> MDPRETAIGLVRYVTENAAKDFDGESIAAIIYRLRVVENYVSSDVDIICEAMRILIKKLVNLPPITFSPDVWMPIMTSITEGAIEPQWRIMMESIDISKFSSTSSNFVHMDSITASSTKCSEQITSICKGFALEFGLTRRLFSAIWNTDLEETARKMMNQEWDSVKIDSSPDSAKQAAGLIEKSIFDLFSEMKDHETFANELYYAALARILNNSRRLQENKKPAIQDSEDISFYESSLHIYDELIKKLWPHLSKKDPNVKKNTLIIFEKLISLSPTDVLVQRITEKFIDSCEWLKISGEEICTSMEPRLWKIVGSLVSRILDLKKTIPYEIVSYAIAVHITQEVTLASPEVSDCGPDSFDSTCDQPSNMKERFLRHMVDSYFQTRSSLLSIIQFLRTAKSSEEIVQFMRVFYPELVFGNETLITHAAIEMLRESASHHSIKADDFISIVLSVIDAPAIVRIIDVISCIKDEKVRKEAVEKTIIRMANDLEDEDQKREGYVNHLHENGSFWNDIAKYADASILDKAGKRFVEVSVDSMDIRSSVLATDIFLTILKLKLTSEAEREPESCVICNVSYSNIKIDLEKWNKMGNILVECNMVKRSKSEALPLFTIHQLENIDLPMRDLVYVVTQMKFLDTKEGMELHRKFYDGLPGVNVIFEKFMSKSHKIELCMKLLDEFAKIIAINEKSLIFSLDHENILDWLEEIGVLDSPQITEKLVDICFSIEVWDVLTLLQLDGPECHYWDLQMFGRFWKTSLMDLLDEKMMKKVNEKMGSILKEQYDKQSHVAKATREKRSNGKFPNRPKVADWEEQLLLMHNRIAGHLTKKKVEDFADESTQKFTWLLGVCSGQMSYKKEVAVDAEKILSRLYPDAEKRNEVLYHFGVSSILKGLDRPRGKLSLHILFMQIYLDLVQIDSKSWKIDDSVQKLSRRLGGFNEWLMIVDEEKREDDGGFRIYIVLNLSHYFWELLEGCKASQVVDAHAILKIRKFAEVLASILDKITFWPNPKLHAYYYIAQFLEPLETIFHFPEIAEQNRKVIESFFKQLFDKLLEQKYQEGLLQDTKLIIQKTDKYLSSSLNLFNEYNTQEPSKIYPVNEIFSLFCRYGSENVHLYCLKMIKKSLQTLASNILEHEHILKGEVCIETELQKRLVCDAVLLTEFFGYFSCIYAQVSENQPSEHDDVAKAFMLLDSDIHLKTKSRKRSTQNSVAVGSHRHQTAENMDLNFCTYKSTGRAYVTQHWYNCYTCNMMESEGVCSVCAINCHRGHDLAYSKKGSFFCDCGEKKCGAMQGIYHLPNSMYSLRGQLPEKNGDKTLPKIRNVFEHRFENLNSNCCDELKSALNDVQEEFKEVQDDLEQILEAVDFANQKALQVTEERLAVLESFNDMDDVIISEKEKFIEPLESGHFLPTRRDDLPVQELRVASSQHKIRELSDIIKLDDGTELLVLIPESIQTCLQLHYMDTRTNLIQGMHALRTETEQIPFNARSLHVSGNRLVVCGQYEFFALRFSPQGDVIDRAHIKLLENGASSSMNNNPVVRAKFCREIESDKRRRQLIAVATMQYIRIYDLTLHETNFVEEMVLPAGNVEDVEIINQEDGNVRILVLSSSGYLYEHNISVFNAENNSIFLTNVVNTPGMDMNGDGVSLHYSSTFNLLFVSLENGAFVAQLPEPTGNSTAPIYDWKHLNIKNPVDAWKETSGIIACLSTNCNHQVNYFHPTVGKILLQKTSVKRSIMTYFLMTSAKNQSVYSVLIYPNVPTCEIWETSWNNVHDLWIDDVPTERYAVEVVEQKSTQIPIDRDELVLLAEQCEQIRTVDWNCREIGMFYTHEELNNRLSSSDSLPITLIQQTHFKLSARITNFRQIVRMIRVEVEGNTGPEYLKIGTTRYSISSRGPKTFDLRLSREESLALDHRDITIEVIPRSNQNRVTLKSLRLLGCDRSAMDEIQPRYERQPILTNSNKLVYSILEFATLSGLEWAGNMAKKHLSRKLNHPAVCSVSTRAIVKCHPSVDEELFKIIDGAYLQEWKALIDWTESEGFGEMRLHHVEQLLDRMEAVRTRWPYFVKSLKREFGTVTSFVELMRNEMKRMPLHRCQMMAQAIVKIVFGLLSNGTNEAEQLIHVFLNIFTDQDTYHLANDMRSAVQETISRFENALKEEKKLMVEHENMDKESVLRIKNYGFSPFYGAPRIIAKTPESMLIAKIAETIPIDSEENFKWLEQLISMILEKLTRSNSTVTWQNLSDSPSYNLSRVLASCLAICDPVIIRNHFSRLIHIIKYDVEKIFPMSEKSYSNYSLLRSVELLLFVCLEKRGDESKENQEMLDSIV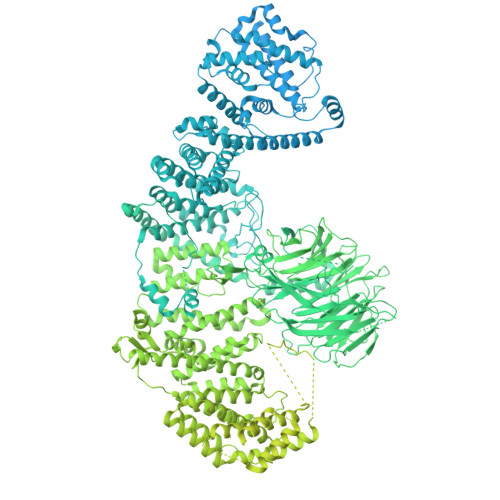HDLQAVGIRNLCLKILEKVIPHWKDRGPSTFSRNSAESRKVWLPHVPLVSSSANPPNTSIMNWPSTSEDSYIIACTDLILLIPQHLQELDRRKSVPRDDQWIQKLCQLASLSSGCSAYRQCKKLLLAMCHNDENKYKIMRDKYKMQDLLQQLVKKYLDVSKEVGGHQQLTEIVDVLASITKLALIRPDMWRDVCSTHTTWLLRLACYTTDVVASQVVELLIVAVRDSSVGGQLSIQLADSIVEAENGEFIEKIIKRFLIGRDEQLRWTLHGMLRSVIQLASRQNQCILVKKLYNTIYPLAANLGVQGAQLVDLIATYAPRVFSSTELVAMTQSEISTIEKIRNTLNGDGYQGMYKLMSDLGLGWKSINFDRNPCLVCFTSKGSHDVVKMTSIKSDIRYSANTIIYKLISNYEVSKVTIKLTELKKSKSIKKVSLYYSAKSVESVDLKLHPELWRKCAMVTVAENETVINLSLAVPVVTSSLIVEFEEVVDHRGSSQLHCPRCTVPVRTHSGVCESCGENAFQCAKCRAINYVEKEPFLCQSCGFCKYAQISLFVVCRALPGAQHITCDAERGQCVQEITQLLIKMETTKTKLTGYRAACESLYLRNRPLPPYKLHVENNHTSEFFDANGTMNIEQLPFQSITMPMNNLAVAIRTLHSELCQQTQQLMYLHEELNRYDHASEVSVVFHKPQNISYYSTGQSCFGCLCNQLLHSVALLHSSCDDENALNLILSSDSLIEKLGVLAQTYETLREEVEELLVRLMFDRLDVTTKVEKLIHTGDINLSVMVKSLMYAADPTWQQKLKLLIRLAMDKRDENCCLQALMVLSKYLEATKSVTLDERKKIKLTPNKNITKWLTTDEEWKDCFSVASTSTAPTKSLPSNPYQWITDCLFSQWMSVRSAANQLLVNLSRQQFHEPVALLILCENMSKLSDVPSSVCDQFMCSAHTIIDSSVNTKARLFVQQFHVYLIKRIHEECAKLHEQSVNLLSDNMFGERLRCFVELLSLLLSGSNVENVLLKAGADDLLIFLLHSTIFLKRIMTRRTRATDSSRIALEKLLKRVSCRDGTKLMSVCVESLKLVKDTSTLGIIVGVMMEIMDPQQETEESFLIQIEKDIAQEDFLQGRMTHNPYNSSDPGMGPLMRDIKNKICRDTEMIALMEDDNGMELLVNGNIISLSLSVRDVYDRLWKRSNNGSPMLIVYRMRGLMGDAVETFIENFGVADNSEADDEEDEQLVRMTHCLMECGGIDKLMDLLTTNVDSSSGRFLLCYLRKIFERIVKIPIGRKILVQRRMVERMMSVIRTCCADPTNESKVLIGMELYKVVEFVVSDKHVQDILGGIREDDAMWWFDLFEKRGNEEGSVTELHRKTAQILDQMTMSIGNIVLGNDASEGVLVKMYEKVLKWEQIDSGAPPSGATDHQNRSRITKKDQIMLMTEQLATITSNIISSAHGIRLKQKILDSGVISSTCNYLTKDLPNLYQPTESPEWKVFLARPSLKLILTLLAGLARGHQASQKEIAKTTLKLMHRLEQVASDNSIGTLAENVIEALNEDEEVRNQIKLVRDETEKKKKQMAMLNREKQLTKMRMKVGTGGQIKVSSRTLHNEPSIDDSDSLPCCICRESVISGDKSAGVYAFAAIDPDSGKTSTVSMMVMVHFNCHKDAIRGGGGRAADEWTRSKLHNAGAKCNVITPISMGVVIGDAWIDALHRFENDVGRVSGLAHGVVNRNFVFVDICNLIDRFIYKRSFSNQSEGGGRESNMQYLAILHLLGITLPADAELEISAPNHRLIAFLFTELTADSWNDQRNDVLRAGINDAQTNGAPATWDGFKPTLMTWAFVDAYFNKVIKITGEDRLEWLREHLVETINKTRGFVDDFDSNILPCEDVAEFCDVTGAPIDDVNLFLAGGPPQGSLEVLFQGPAEAAAKEAAAKEAAAKEAAAKALEAEAAAKEAAAKEAAAKEAAAKAHHHHHHHHHH> MTLEKFVDALPIPDTLKPVQQSKEKTYYEVTMEECTHQLHRDLPPTRLW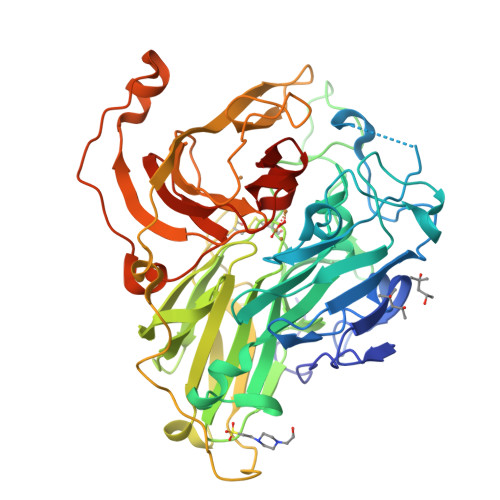GYNGLFPGPTIEVKRNENVYVKWMNNLPSTHFLPIDHTIHHSDSQHEEPEVKTVVHLHGGVTPDDSNGYPEAWFSKDFEQTGPYFKREVYHYPNQQRGAILWYHDHAMALTRLNVYAGLVGAYIIHDPKEKRLKLPSDEYDVPLLITDRTINEDGSLFYPSAPENPSPSLPNPSIVPAFCGETILVNGKVWPYLEVEPRKYRFRVINASNTRTYNLSLDNGGDFIQIGSDGGLLPRSVKLNSFSLAPAERYDIIIDFTAYEGESIILANSAGCGGDVNPETDANIMQFRVTKPLAQKDESRKPKYLASYPSVQHERIQNIRTLKLAGTQDEYGRPVLLLNNKRWHDPVTETPKVGTTEIWSIINPTRGTHPIHLHLVSFRVLDRRPFDIARYQESGELSYTGPAVPPPPSEKGWKDTIQAHAGEVLRIAATFGPYSGRYVWHCHILEHEDYDMMRPMDITDPHK> PKISLQIPIKLKSVLVDDWEYVTKDKKICRLPADVTVEMVLNKYEHEVSQELESPGSQSQLSEYCAGLKLYFDKCLGNMLLYRLERLQYDELLKKSSKDQKPLVPIRIYGAIHLLRLISVLPELISSTTMDLQSCQLLIKQTEDFLVWLLMHVDEYFNDKDPNRSDDALYVNTS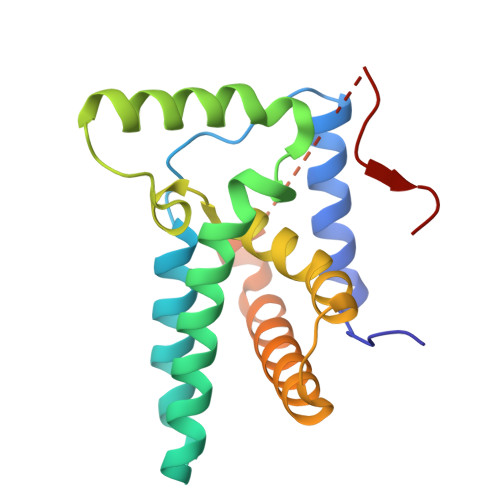SQYEGVALGM> SMQSSKRSSRSVEDDKEGHLVCRIGDWLQERYEIVGNLGEGTFGKVVECLDHARGKSQVALKIIRNVGKYREAARLEINVLKKIKEKDKENKFLCVLMSDWFNFHGHMCIAFELLGKNTFEFLKENNFQPYPLPHVRHMAYQLCHALRFLHENQLTHTDLKPENILFVNSEFETLYNEHKSCEEKSVKNTSIRVADFGSATFDHEHHTTIVATRHYRPPEVILELGWAQPCDVWSIGCILFEYYRGFTLFQTHENREHLVMMEKILGPIPSHMIHRTRKQKYFYKGGLVWDENSSDGRYVKENCKPLKSYMLQDSLEHVQLFDLMRRMLEFDPAQRITLAEALLHPFFAGLTPEERSFHT

Increased kinase activity of leucine-rich repeat kinase 2 (LRRK2) is associated with Parkinson’s disease (PD). Here, to our knowledge, we present the first type II kinase inhibitors that target LRRK2. We designed these inhibitors with a combinatorial chemistry approach fusing selective LRRK2 type I and promiscuous type II inhibitors using iterative cycles of synthesis supported by structural biology and activity testing. Type II inhibitors stabilize the inactive/open kinase conformation, reaching into the far back pocket of the kinase active site and disrupting a critical salt-bridge by releasing the regulatory αC helix.

The initial compound 28 obtained from this chemical series, named RN129, outperformed all previously designed and tested hybrid type II inhibitors both in stabilizing LRRK2KW and in inhibiting LRRK2 kinase activity (IC50 = 59.7 nM). Unfortunately, RN129 (28) was not only, by far, the most potent LRRK2 inhibitor designed using our hybridization approach, but also the most promiscuous one, showing high thermal stabilization of 49% of the kinases screened. To elucidate the binding mode of RN129 (28) and to inform future design strategies, we obtained a co-crystal structure of RN129 (28) with one of its potent off-targets, CDC-like kinase 3 (CLK3), a kinase that has been crystallized routinely in our group. Our structure revealed that RN129 (28) has a canonical type II binding mode that has not been described for CLK3 previously. As expected, the 7H-pyrrolo[2,3-d]pyrimidine moiety of RN129 (28) formed two hydrogen bonds with the hinge of CLK3. The linking phenyl ring formed a π-π interaction with the phenylalanine F236. The urea was located between the αC helix and the DFG motif, with the bulky tail of the molecule extending into the far back pocket. The hinge of CLK3 contains a leucine residue (L238) that is also present in LRRK2, whereas most human kinases have larger phenylalanine or tyrosine residues at this position. Therefore, we hypothesized that developing the inhibitor toward this residue would improve selectivity.> MTRYYCEYCHSYLTHDTLSVRKSHLVGKNHLRITADYYRNKARDIINKHNHKRRHIGKRGRKERENSSQNETLKVTCLSNKEKRHIMHVKKMNQKELAQTSIDTLKLLYDG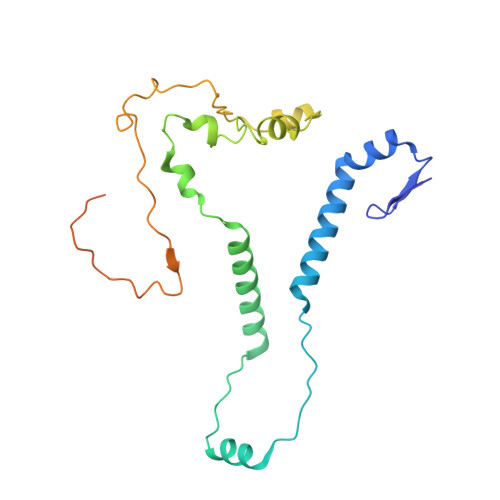SPGYSKVFVDANRFDIGDLVKASKLPQRANEKSAHHSFKQTSRSRDETCESNPFPRLNNPKKLEPPKILSQWSNTIPKTSIFYSVDILQTTIKESKKRMHSDGIRKPSSANGYKRRRYGN> MKYQSQSIALVYFAVALGLFAIQVSGGLLLGWIYVSPNFLSEILPFNIVRMLHTNSLIVWLLLGFMGAAYFVIPEESEREIHSPLLAYLQLAIMVLGTLGVVVTYLFNLFEGNWLLGKEGREFLEQPVWVKMGIVVAALIFMYNISMTVLQGRKTAITNVLLLGLWGLTLLFLFAFYNPSNLALDKMYWWYVVHLWVEGTWELVMASVLAFLMLKLTGVDREIIEKWLYLIVATALFSGILGTGHHYFWIGTPGYWQWIGSIFSALEVVPFFGMMAFAFVMVWKGRKDHPNKAALLWSLGCATLAFFGAGVWGFLHTLHGINYYTHGTQITAAHGHLAFFGAYVSLNLAIFSYAFPILRKRDPYNQVLNMASFWLMAGGMTFMTFVLTFAGTVQTHAQRVQGDYFMDVQDAITIFYWMRFGSGIAVVLGALLFIYAVAVPRKEIISP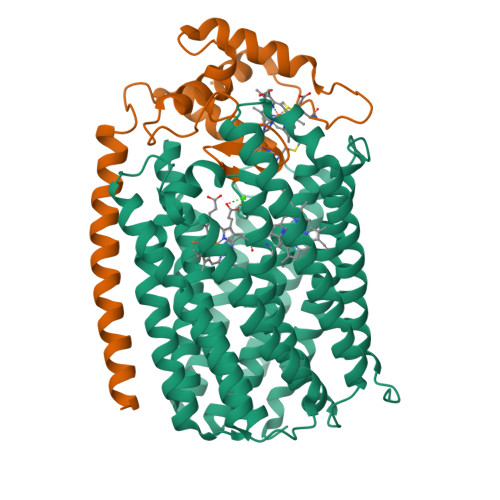SDKQPVAAE;> MRDVLTTSMARNIFYGGSLFFILIFVGLSVHSHRYIVTTSTDAATLTAEVEHGKHLWEIHGCVNCHSILGEGAYFAPELGNVMTRWGVEDDPDAAFEALKGWMDAMPTGIEGRRQMPNFGLNDEEYRALSDFLLWTNTIRNQDWPPNDAG5-IMINO-4-(2-TRIFLUOROMETHYL-PHENYLAZO)-5H-PYRAZOL-3-YLAMINE 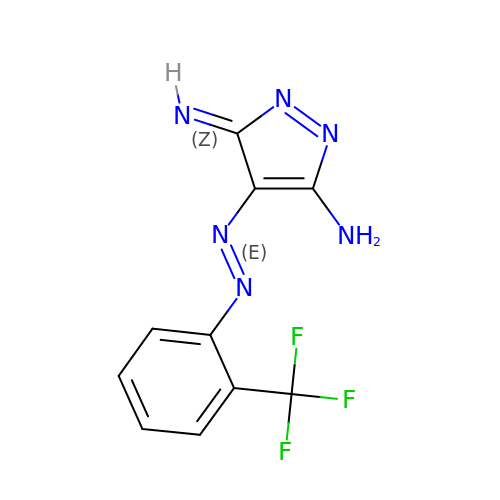| C10 H7 F3 N6 | KJHMEAOMPGLBTJ-LKCQKNGNSA-N>AQTVPYGIPLIKADKVQA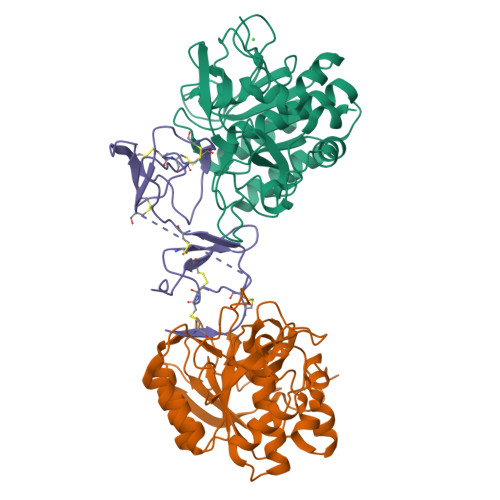QGFKGANVKVAVLDTGIQASHPDLNVVGGASFVAGEAYNTDGNGHGTHVAGTVAALDNTTGVLGVAPSVSLYAVKVLNSSGSGSYSGIVSGIEWATTNGMDVINMSLGGASGSTAMKQAVDNAYARGVVVVAAAGNSGNSGSTNTIGYPAKYDSVIAVGAVDSNSNRASFSSVGAELEVMAPGAGVYSTYPTNTYATLNGTSMASPHVAGAAALILSKHPNLSASQVRNRLSSTATYLGSSFYYGKGLINVEAAAQ[2x];> KACTRECGNLGFGICPRSEGSPLNPICINCCSGYKGCNYYNSFGKFICEGESDPKRPNACTFNCDPNIAYSRCPRSQGKSLIYPTGCTTCCTGYKGCYYFGKDGKFVCEGESDEPKANMYPVM> SNRTILVTGATGTQGGATVRALLARGRPVRALVRDPGTDAARALAAAGVSLVTGDLNDQASLRAAMADVHGVFSVQTFMTPGGLGAELRQGRAVADAAAATGVR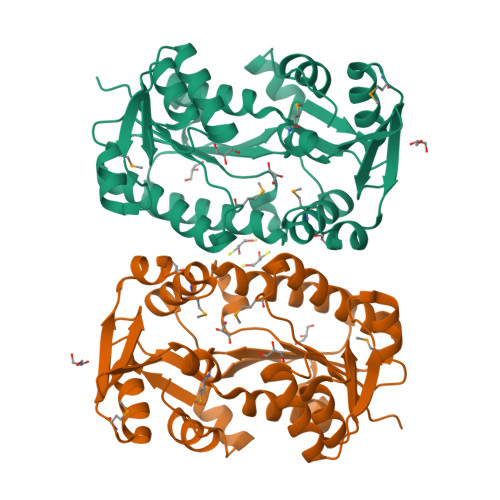HVVYSSVGGADRASGVPHFETKWTIERHLRSLGVPTTVLRPTFFMDNFAAWGPQAVDGTLVVRLPLKPQTRVQLIAAEDIGVFAATAFDDPDTYVGAALELAGDELTGPELAARFGELAGMPARFEERSLDEAAADPWIPYSHEIAVMFEWFQTDGYAADIAALRARHPGLRTFADWLRAIGWRVP>[2x]MPNIKIFSGSSHQDLSQKIADRLGLELGKVVTKKFSNQETCVEIGESVRGE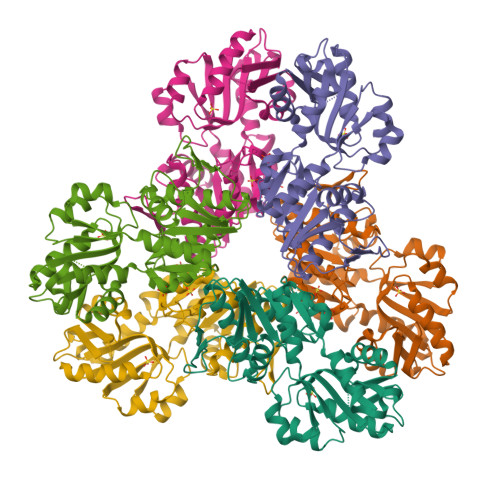DVYIVQSGCGEINDNLMELLIMINACKIASASRVTAVIPCFPYARQDKKDKSRAPISAKLVANMLSVAGADHIITMDLHAAQIQGFFDIPVDNLYAEPAVLKWIRENISEWRNCTIVSPDAGGAKRVTSIADRLNVDFALIHKERKKANEVDRMVLVGDVKDRVAILVDDMADTCGTICHAADKLLSAGATRVYAILTHGIFSGPAISRINNACFEAVVVTNTIPQEDKMKHCSKIQVIDISMILAEAIRRTHNGESVSYLFSHVPLLEHHHHHH> MDSRDSEVLIHPSAVVHPNAVIGKGVSVGPYCTIGSSVKLGNGCKLYPSSHVFGNTELGESCVLMTGAVVGDELPGYTFIGCNNIIGHHAVVGVKCQDLKYKHGDECFLCIGNNNEIREFCSIHRSSKPSDKTVIGDNNLIMGSCHI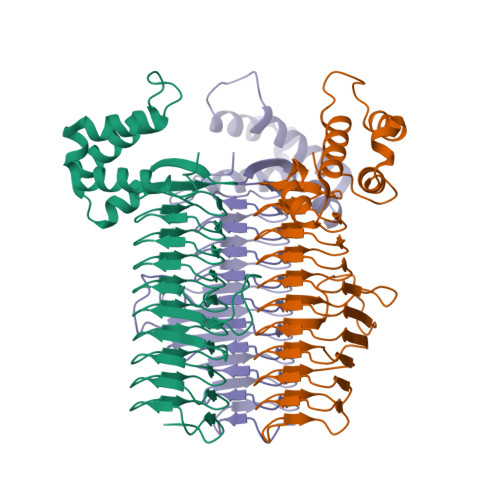AHDCKIGDRNIFANNTLLAGHVVVEDNTHTAGASVVHQFCHIGSFAFIGGGSVVSQDVPKYMMVAGERAELRGLNLEGLRRNGFTMSEMKSLRAAYRKIFMSTETVSLSFEERLTELEQDQELYSVPAVSAMLQSIRDSFTESRRGICKFRQWLDSTT> ESLPDLKIEKLDEGVYVHTSFEEVNGWGVVPKHGL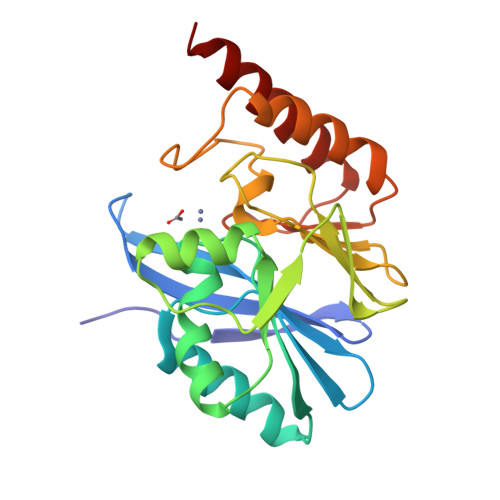VVLVNAEAYLIDTPFTAKDTEKLVTWFVERGYKIKGSISSHFHSDSTGGIEWLNSRSIPTYASELTNELLKKDGKVQATNSFSGVNYWLVKNKIEVFYPGPGHTPDNVVVWLPERKILFGGCFIKPYGLGNLGDANIEAWPKSAKLLKSKYGKAKLVVPSHSEVGDASLLKLTLEQAVKGLNESK>[2x]HMLGKIALEEAFALPRFEEKTRWYASLFSTDAETHVKEITDINKIRIEHADKHGVGYQILSYTAPGVQDIWDPVEAQALAVEINDYIAEQVRVNPDRFGAFATLSMHNPKEAADELRRCVEKYGFKGALVNDTQRAGPDGDDMIFYDNADWDIFWQTCTELDVPFYMHPRNPTGTIYEKLWADRKWLVGPPLSFAHGVSLHVLGMVTNGVFDRHPKLQIIMGHLGEH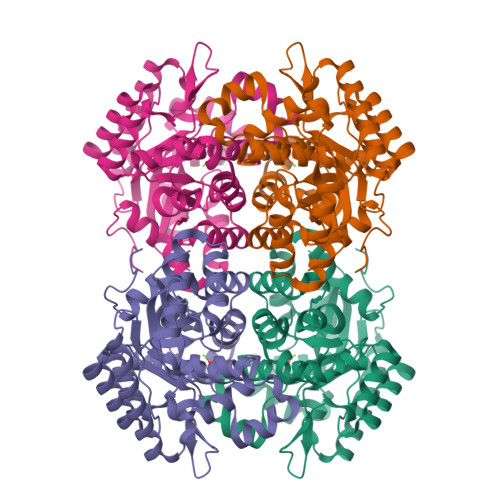VPFDMWRINHWFEDRKKLLGLAETCKKTIRDYFAENIWITTSGHFSTTTLNFCMAEVGSDRILFSIDYPFETFSDACEWFDNAELNGTDRLKIGRENAKKLFKLDSYKDSSA> MVQDTGKDTNLKGTAEANESVVYCDVFMQAALKEATCALEEGEVPVGCVLVKADSSTAAQAQAGDDLALQKLIVARGRNATNRKGHGLAHAEFVAVEELLRQATAGTSENIGGGGNSGAVSQDLADYVLYVVVEPCIMCAAMLLYNRVR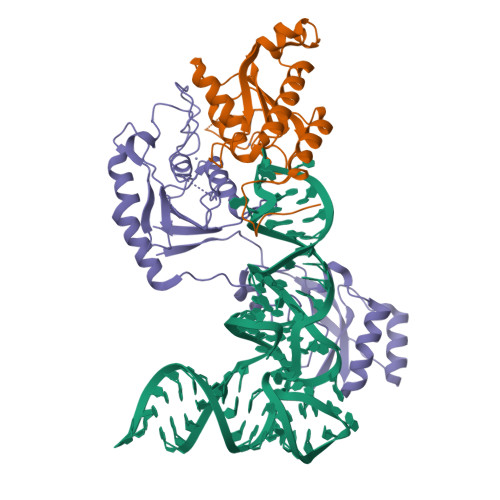KVYFGCTNPRFGGNGTVLSVHNSYKGCSGEDAALIGYESCGGYRAEEAVVLLQQFYRRENTNAPLGKRKRKD;> GPDSMEEVVVPEEPPKLVSALATYVQQERLCTMFLSIANKLLPLKPHACHLKRIRRSSATRVATAPMDGFAGGVICDKRDSSVATSTISDGCERNSAALGTPAAEKSHVLELLLSVGGPVDSSALKELESAADTTVAVHRVWVPDRAPRSSAEEWTKWCQIWPFATPKPRVPTQLSECEVGSIQRIFRTVVMPLAKRLRTDETLGIAAVLVDPSDGYRVLVSSGEEHALKRGNSAACLGYVSNSGCRKSNRVVLDHPVTFVLKEVTRKQCKDREVEGDASYLANGMDMFVSHEPCVMCSMALVHSRVRRVFYCFPNPVHGGLGSTVSIHAIQELNHHFRVFRCDSRWLSDPEGVSSDHDNPYWEDLTVP(propan-2-yl)benzene | C9 H12 | 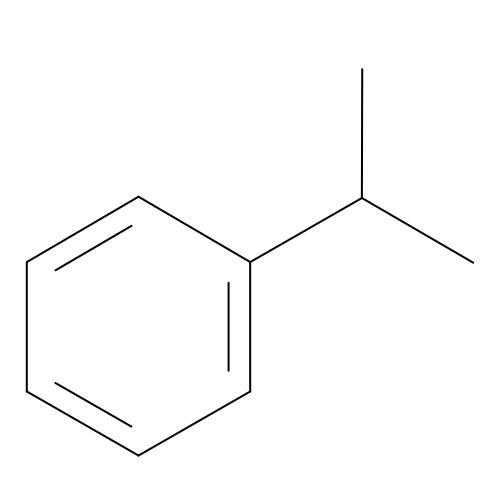RWGFKTVRMDUZSP-UHFFFAOYSA-N>MEEVVIAGMSGKLPESENLEEFWANLIGGVDMVTADDRRWKAGLYGLPRRMGKLKDLSRFDASFFGVHSKQANTMDPQLRMLLEVTYEAIVDGGINPASLRGTSTGVWVGVSSSDASEALSRDPETLVGYSMIGCQRAMMANRLSFFFDFKGPSITIDTACSSSLLALQSAYQAIRGGECSAAVVGGLNVLLKPNSSLQFMKLGMLSQDGTCRSFDAEGTGYCRAEAVVAVLLTKKSLARRVYATILNAGTNTDGSKEQGVTFPSGDVQEQLIRSLYAPAGPDPESLEYIEAHGTGTKVGDPQELNGIVNALCATRREPLLIGSTKSNMGHPEPASGVAALIKVLLSLEHGVWAPNLHYHTPNPEIPALQDGRLQVVDRPLPIRGGNVGINSFGFGGSNVHVILQPNSRPAPPPAQHAALPRLLQASGRTLEAVQTLLEQGLRHSRDLAFVGMLNEIAAVSPVAMPFRGYAVLGGEAGSQEVQQVPGSKRPVWFICSGMGAQWQGMGLSLMRLDRFRDSILRSDQALKPLGLRVSDLLLSTDEAVLDDIVSSFVSLTSIQIALIDLLTSLGLQPDGIIGHSLGEVACGYADGCLTQEEAVLSSYWRGYCIKEANVLPGAMAAVGLSWEECKQRCPPGIVPACHNSKDTVTISGPQAAMSEFLQQLKREDVFVKEVRTGGIAFHSYFMESIAPTLLRQLRKVILDPKPRSKRWLSTSIPEAQWQGSLARTFSAEYSVNNLVSPVLFQEALQHVPAHAVVVEIAPHALLQAVLKRSLESSCTIIPLMKKDHRDNLEFFLSNVGRLHLAGVSVNPNGLFPPVEFPAPRGTPLISPHIKWDHSQAWDVPSAADFPSGSSCSSVAVYKFDVSPESPDHYLVDHCIDGRVLFPGTGYLWLTWKTLARALSQNLEETPVVFEDVTLHQATILPKTGTVSLEVRLLEASHAFEVSDSNGSLIASGKVYQWESPDPKLFDTRAAVDPADSTAEFRLSQGDVYKDLRLR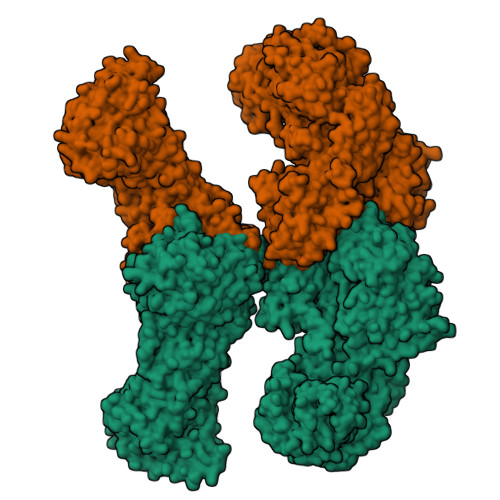GYDYGPFFQLVLESDLEGNRGRLQWNDSWVSFLDAMLHMSILAPGQLGLYLPTRFTSIRIDPVTHRQKLYTLQDTTQAADVVVDRNLNTVVAGGALFLGAHSSVAPRRPQEHLKPILEKFCFTPHVESGCLAGNTALQEELQLCRGLAQALQTKVAQQGLKMVVPGLDGAQAPREAPQQSLPRLLAAACQLQLNGNLQLELGQVLAQERPLLCDDPLLSGLLDAPALKACVDTALENMASPKMKVVEVLAGDGQLYSRIPALLNTQPVMDLDYTATDRNPQALEAAQAKLEQLHVTQGQWDPANPAPGSLGKADLLVCNCALATLGDPAVAVGNMAATLKEGGFLLLHTLLAGHPLGEMVGFLTSPEQGGRHLLSQDQWESLFAGASLHLVALKRSFYGSVLFLCRQQTPQDSPVFLSVEDTSFRWVDSLKDILADASSRPVWLMAVGCSTSGVVGMVNCLRKEPGGHRIRCVLVSNLSSTSPAPEMHPSSSELQKVLQGDLVMNVYRDGAWGAFRHFPLEQDRPEKQTEHAFVNVLSRGDLSSIRWVCSPLHYALPASCQDRLCSVYYTSLNFRDVMLATGKLSPDSIPGKWLTRDCMLGMEFSGRDASGRRVMGMVPAEGLATSVLLLQHATWEVPSTWTLEEAASVPIVYTTAYYSLVVRGRMQPGESVLIHSGSGGVGQAAIAIALSRGCRVFTTVGSAEKRAYLQARFPQLDETCFANSRDTSFEQHVLRHTAGKGVDLVLNSLAEEKLQASVRCLAQHGRFLEIGKFDLSNNHALGMAVFLKNVTFHGILLDSLFEEGGATWQEVSELLKAGIQEGVVQPLKCTVFPRTKVEAAFRYMAQGKHIGKVVIQVREEEQGPAPRGLPPIALTGLSKTFCPPHKSYVITGGLGGFGLQLAQWLRLRGAQKLVLTSRSGIRTGYQARQVREWRRQGVQVLVSTSNASSLDGARSLITEATQLGPVGGVFNLAMVLRDAVLENQTPEFFQDVSKPKYSGTANLDRVTREACPELDYFVIFSSVSCGRGNAGQANYGFANSAMERICEKRRHDGLPGLAVQWGAIGDVGVVLETMGTNDTVIGGTLPQRIASCLEVLDLFLSQPHPVLSSFVLAEKKAAAPRDGSSQKDLVKAVAHILGIRDVASINPDSTLVDLGLDSLMGVEVRQILEREHDLVLSMREVRQLSLRKLQELSSKTSTDADPATPTSHEDSPVRQQATLNLSTLLVNPEGPTLTRLNSVQSAERPLFLVHPIEGSITVFHGLAAKLSIPTYGLQCTGAAPLDSIQSLASYYIECIRQVQPEGPYRIAGYSYGACVAFEMCSQLQAQQSATPGNHSLFLFDGSHTFVLAYTQSVRAKMTPGCEAEAEAKAMYFFVQQFTDMEQGKVLEALIPLQGLEARVAATVDLITQSHAGLDRHALSFAARSFYQKLRAAENYWPQATYHGNVTLLRAKTGGAYGEDLGADYNLSQVCDGKVSVHVIEGDHRTLLEGSGLESILSIIHSCLAEPRVSVREG[2x]>[2x]NDPSQVKTLQEKAGKGAGTVVAVIDAGFDKNHEAWRLTDKTKARYQSKEDLEKAKKEHGITYGEWVNDKVAYYHDYSKDGKTAVDQEHGTHVSGILSGNAPSETKEPYRLEGAMPEAQLLLMRVEIVNGLADYARNYAQAIRDAINLGAKVINMSFGNAALAYANLPDETKKAFDYAKSKGVSIVTSAGNDSSFGGKTRLPLADHPDYGVVGTPAAADSTLTVASYSPDKQLTETVRVKTADQQDKEMPVLSTNRFEPNKAYDYAYANRGTKEDDFKDVKGKIALIERGDIDFKDKIAKAKKAGAVGVLIYDNQDKGFPIELPNVDQMPAAFISRKDGLLLKDNPQKTITFNATPKVLPTASGT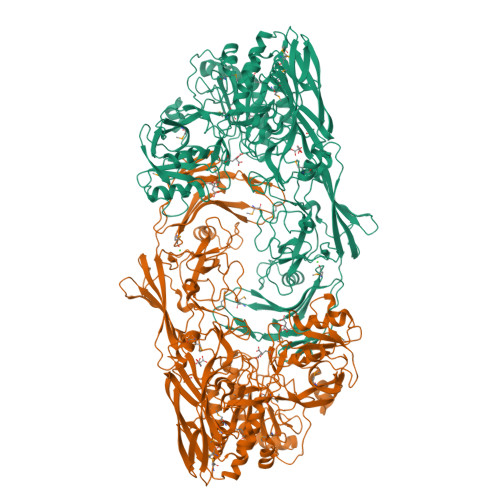KLSRFSSWGLTADGNIKPDIAAPGQDILSSVANNKYAKLSGTSMSAPLVAGIMGLLQKQYETQYPDMTPSERLDLAKKVLMSSATALYDEDEKAYFSPRQQGAGAVDAKKASAATMYVTDKDNTSSKVHLNNVSDKFEVTVNVHNKSDKPQELYYQATVQTDKVDGKHFALAPKVLYETSWQKITIPANSSKQVTVPIDASRFSKDLLAQMKNGYFLEGFVRFKQDPTKEELMSIPYIGFRGDFGNLSALEKPIYDSKDGSSYYHEANSDAKDQLDGDGLQFYALKNNFTALTTESNPWTIIKAVKEGVENIEDIESSEITETIFAGTFAKQDDDSHYYIHRHANGKPYAAISPNGDGNRDYVQFQGTFLRNAKNLVAEVLDKEGNVVWTSEVTEQVVKNYNNDLASTLGSTRFEKTRWDGKDKDGKVVANGTYTYRVRYTPISSGAKEQHTDFDVIVDNTTPEVATSATFSTEDRRLTLASKPKTSQPVYRERIAYTYMDEDLPTTEYISPNEDGTFTLPEEAETMEGATVPLKMSDFTYVVEDMAGNITYTPVTKLLEGH> GASPASTNPAHDHFETFVQAQLCQDVLSSFQGLCRALGVESGGGLSQYHKIKAQLNYWSAKSLWAKLDKRASQPVYQQGQACTNTKCLVVGAGPCGLRAAVELALLGARVVLVEKRIKFSRHNVLHLWPFTIHDLRALGAKKFYGRFCTGTLDHISIRQLQLLLLKVALLLGVEIHWGVKFTGLQPPPRKGSGWRAQLQPNPPAQLASYEFDVLISAAGGKFVPEGFTIREMRGKLAIGITANFVNGRTVEETQVPEISGVARIYNQKFFQSLLKATGIDLENIVYYKDETHYFVMTAKKQCLLRLGVLRQDLSETDQLLGKANVVPEALQRFARAAADFATHGKLGKLEFAQDARGRPDVAAFDFTSMMRAESSARVQEKHGARLLLGLVGDCLVEPFWPLGTGVARGFLAAFDAAWMVKRWAEGAGPLEVLAERESLYQLLSQTSPENMHRNVAQYGLDPATRYPNLNLRAVTPNQVQDLYDMMDKEHAQRKSDEPDSRKTTTGSAGTEELLHWCQEQTAGFPGVHVTDFSSSW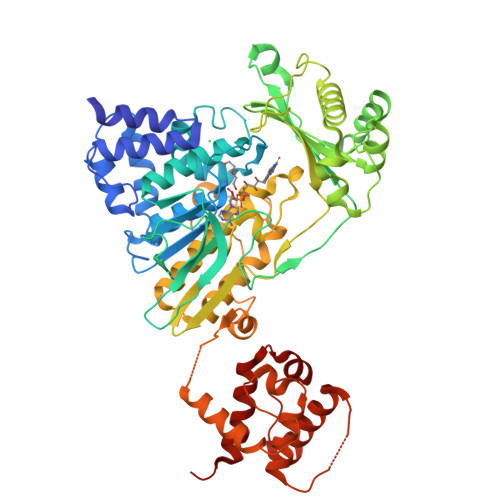ADGLALCALVHHLQPGLLEPSELQGMGALEATTWALRVAEHELGITPVLSAQAVMAGSDPLGLIAYLSHFHSAFKNTSH> MGHHHHHHENLYFQGYNTVEEQKMRHLRFENLTEEQLKRLAKILTENLKGGEVVILSGNLGAGKTTFVKGMIRAIGLDEKMVKSPTFTLMNVYPGLKTIYHLDLYRLQ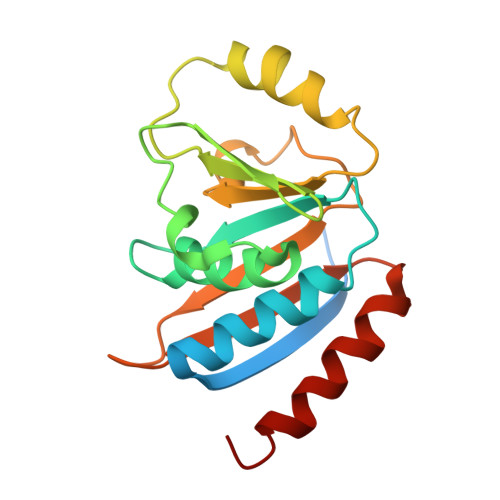DTDFLSLDVEDILEDEDGIMVVEWGDLFDGFWPEDSIKVKIEIADESHRNVEILIPEEVNFLVEKIERYRKELQNT> MASNEARYV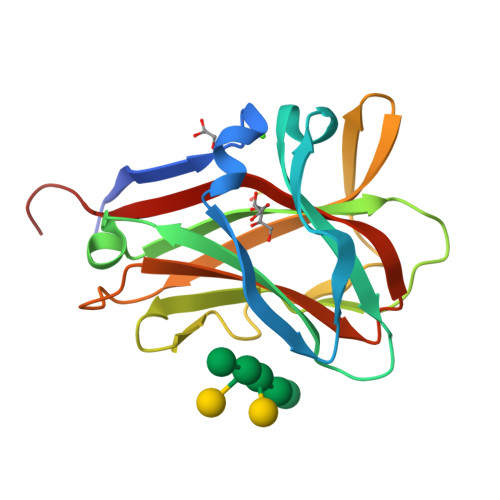LAEEVDFSSPEEVKNWWNSGTWQAEFGSPDIEWNGEVGNGALQLNVKLPGKSDWEEVRVARKFERLSECEILEYDIYIPNVEGLKGRLRPYAVLNPGWVKIGLDMNNANVESAEIITFGGKEYRRFHVRIEFDRTAGVKELHIGVVGDHLRYDGPIFIDNVRLYKRTGGM>WIENIPL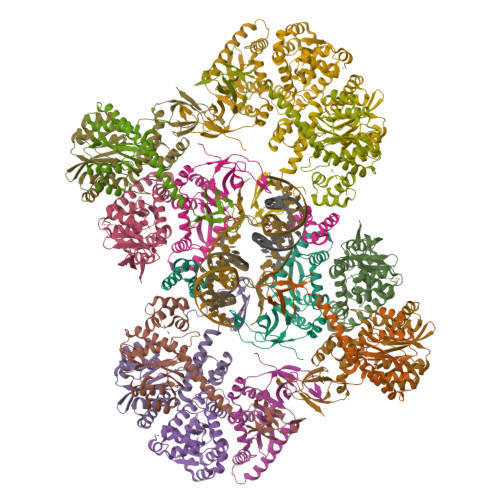AEEEHNKWHQDAVSLHLEFGIPRTAAEDIVQQCDVCQENKMPSTLRGSNKRGIDHWQVDYTHYEDKIILVWVETNSGLIYAERVKGETGQEFRVQTMKWYAMFAPKSLQSDNGPAFVAESTQLLMKYLGIEHTTGIPWNPQSQALVERTHQTLKNTLEKLIPMFNAFESALAGTLITLNIKRKGGLGTSPMDIFIFNKEQQRIQQQSKSKQEKIRFCYYRTRKRGHPGEWQGPTQVLWGGDGAIVVKDRGTDRYLVIANKDVKFIPPPKEIQKE[16x]>MTLEAIRYSRGSLQILDQLLLPKQSRYEAVGSVHQAWEAIRAMKVRGAPAIALVGCLSLAVELQAGAGGPGLAALVAFVRDKLSFLVTARPTAVNMARAARDLADVAAREAEREGATEEAVRERVICCTEDMLEKDLRDNRSIGDLGARHLLERVAPSGGKVTVLTHCNTGALATAGYGTALGVIRSLHSLGRLEHAFCTETRPYNQGARLTAFELVYEQIPATLITDSMVAAAMAHRGVSAVVVGADRVVANGDTANKVGTYQLAIVAKHHGIPFYVAAPSSSCDLRLETGKEIIIEERPGQELTDVNGVRIAAPGIGVWNPAFDVTPHDLITGGIITELGVFAPEELRTALTTTISS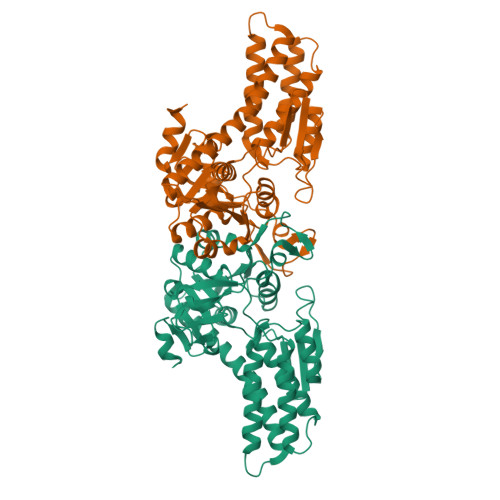RDGTLDGPQM[2x]>[2x]EAEAEFLGSTCSSPLTHGSAAPGDPFWLQNIQHQGIAAFNGNPGGYPVFRNVKNYGAKGDGNTDDTAAIQAAINAGGRCGQGCDSTTTQPALVYFPPGTYKVSSPLVVLYQTQLIGDAKNLPTLLAAPNFSGIALIDADPYLAGGAQYYVNQNNFFRSVRNFVIDLRQVSGSATGIHWQVSQATSLINIVFQMSTAAGNQHQGIFMENGSGGFLGDLVFNGGNIGATFGNQQF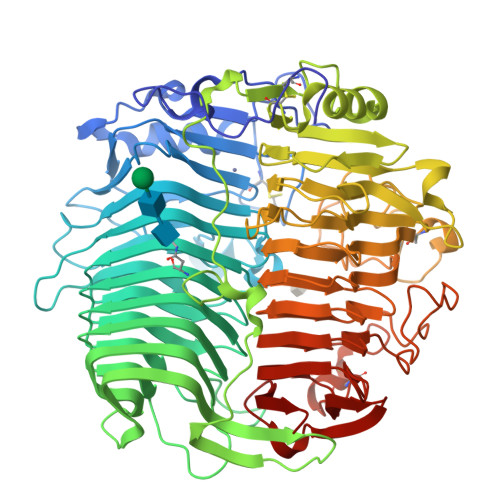TVRNLTFNNANTAINAIWNWGWTFQRITINNCQVGFDLTQGGTSNTGAQGVGAEAIIDAVVTNTQTFVRWSGASSGHLQGSLVLNNIQLTNVPVAVGVKGGPTVLAGGTTTINSWAQGNVYHGTNGNPTFTQGNIANINRPGVLLDSTGRIVSKSHPQYTGYAPSDFVSVRSQGAKGDGHTDDTQAIKNVFAKYAGCKIIFFDAGTYIVTDTIQIPAGTQIVGEVWSVIMGTGSKFTDYNNPQPVIQVGAPGSSGVVEITDMIFTTRGPAAGAIIVEWNVHDPSGQQAAAGAWDTHLIIGGTAQSGLQVGQCPTSGAGGNNCFADFLGLHLTSGSSAYLEGMWVWLADHDLDSGGSQQISLWSNGGIMSESQGPVWLIGTASEHHINYQYFLKNAANHYIGLAQTETPYFQPNPNPPAPFITNSNFDPSQLGQGDAWAMTVQNSHGILVFGAGFYSFFSAYNTGCQSPQNCQNQIVNVDSSSDIAFYSLTTVDTTWQFSVNAQGVINRSNNPNGFADTITAWTRN> MILVGIAVLILLAVFAILYYKQKEKFVVVGKFVEPIPSNPGQDFTLLPMDQTYTFADPVPDTATAFDVVLSRFTDKKAPADLLKGATFPEAAPYTDSEVENISKLALSRVKGPDAPVLSFISVEYAAKGVDNKKNTHYDIAFMVYDQVKNFSLKLVLVAVLDAKNKLWIKKFSSFNSFTPKDKGPKGVENIDETPLAEFIPDF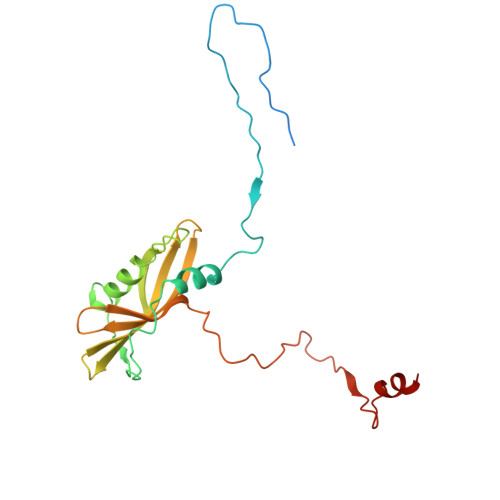VQFSRLYKDNANV N-methyl-8-(piperazin-1-yl)-1,2,3,4-tetrahydro[1,2,3]triazino[4',5':4,5]thieno[2,3-c]isoquinolin-5-amine | C17 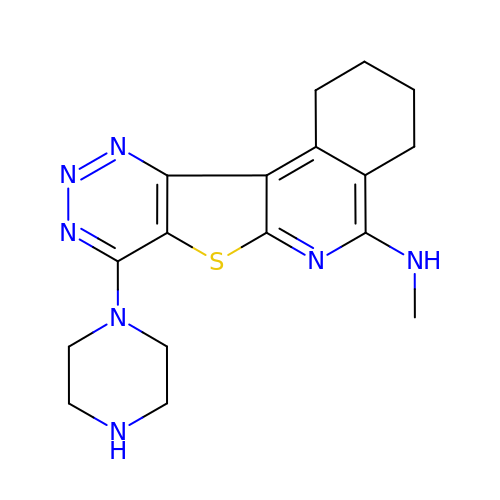H21 N7 S | KOWHYIUBBFEWRP-UHFFFAOYSA-N>MKTIIALSYIFCLVFAGRALVPEKEKDPKYWRDQAQETLKYALELQKLNTNVAKNVIMFLGDGMGVSTVTAARILKGQLHHNPGEETRLEMDKFPFVALSKTYNTNAQVPDSAGTATAYLCGVKANEGTVGVSAATERSRCNTTQGNEVTSILRWAKDAGKSVGIVTTTRVNHATPSAAYAHSADRDWYSDNEMPPEALSQGCKDIAYQLMHNIRDIDVIMGGGRKYMYPKNKTDVEYESDEKARGTRLDGLDLVDTWKSFKPRYKHSHFIWNRTELLTLDPHNVDYLLGLFEPGDMQYELNRNNVTDPSLSEMVVVAIQILRKNPKGFFLLVEGGRIDHGHHEGKAKQALHEAVEMDRAIGQAGSLTSSEDTLTVVTADHSHVFTFGGYTPRGNSIFGLAPMLSDTDKKPFTAILYGNGPGYKVVGGERENVSMVDYAHNNYQAQSAVPLRHETHGGEDVAVFSKGPMAHLLHGVHEQNYVPHVMAYAACIGANLGHCAPAAAAENLYFQGCCPGCC[8x]

HPP patients exhibit hypo-mineralization and osteopenia due to the deficiency or malfunction of tissue non-specific alkaline phosphatase (TNAP), which catalyzes the hydrolysis of phosphate-containing molecules outside the cells, promoting the deposition of hydroxyapatite in the extracellular matrix. Several proteins enriched in the matrix vesicles supply sufficient phosphate for the crystallization of hydroxyapatite, and among them, the TNAP catalyzes the hydrolysis reaction using the pyrophosphate and organic phosphate esters as the substrates, such as pyrophosphate (PPi), pyridoxal phosphate (PLP) and phosphoethanolamine (PEA). The catalytic center of hTNAP is comprised of the catalytic residue S110 and three metal binding sites, one for Mg2+ and two for Zn2+ (1 and 2). The calcium-binding site includes the acidic residues E235, E291, and D306 forming strong static electric interactions with the Ca2+ ion, as well as R223, Y236, and T305 stabilizing the local conformation of the binding pocket.

Crystallization trials showed the crystals of purified hTNAP could grow in both acidic and basic pH conditions diffracting to about 5–10 Å resolution. In both structures determined with hTNAP crystals grown in acidic and basic pH conditions, four TNAP dimers, i.e., protomers A-B, C-D, E-F, and G-H, form an X-shape homo-octamer stabilized with the molecular contacts among protomers B, F, D, and H. The TNAP octamer is maintained with four major interfaces between dimeric TNAPs. Two pairs of dimers, A-B/C-D and E-F/G-H, first form two tetramers with a large interface (interface L) comprising residues from helices 1–3, 18, and 20 via a series of static electric interactions and hydrogen bonds among H79 and D25/D31, E35, and H78, K38/K45 and E311, S364-S368, and T366-T366 from the contacting protomers. The tetramers A/B/C/D and E/F/G/H then dimerize to form the octamer with two small interfaces (interface S) comprising H7, H14, and some loops. Interestingly, multiple HPP-associated mutation sites were mapped in interface L and S, including D156, K264, A492, and C497 from interface S and Y28, E311, T366, and S368 from interface L. The crystallographic analysis of hTNAP has uncovered an unexpected octameric structure that has not been observed in other previously reported AP structures. However, the disruption of the hTNAP function resulting from mutations on the octameric interface implies that hTNAP may be stabilized by octamerization, which prevents the interfaces from exposure. The conserved catalytic residue S110 was solved as the unphosphorylated form in all the protomers, which serve as a nucleophile in attacking the phosphorous. However, once released into circulation upon the PIPLC cleavage, TNAP can polymerize into its oligomeric form.> GPLGSTAFRKFYERGDFPIALEHDSKGNKIAWKVEIEKLDYHHYLPLFFDGLCEMTFPYEFFARQGIHDMLEHGGNKILPVLPQLIIPIKNALNLRNRQVICVTLKVLQHLVVSAEMVGKALVPYYRQILPVLNIFKNMNVNSGDGIDYSQQKRENIGDLIQETLEAFERYGGENAFINI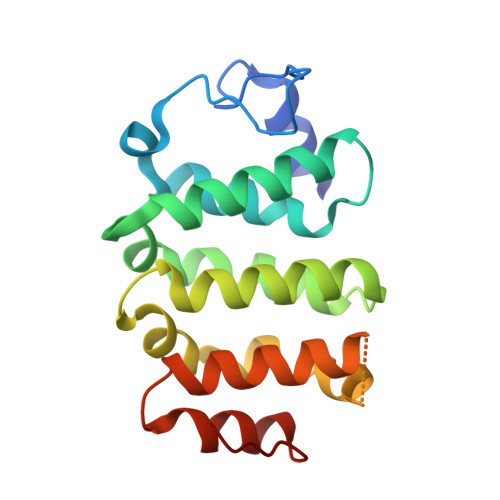KYVVPTYESCLLN Here, we present single-crystal X-ray structures of CheY from Pyrococcus horikoshii (PhCheY) in two different crystal forms, and the protein purification, crystallization and X-ray data collection of CheF (PhCheF). CheA autophosphorylates and subsequently donates the phosphate to CheY, yielding phosphorylated CheY (CheY-P; Garrity & Ordal, 1997; Bischoff et al., 1993; Rudolph & Oesterhelt, 1995; Rudolph et al., 1995). The concentration of CheY-P determines the switching frequency of the flagellum or archaellum, respectively. We observe PhCheY to have a domain-swapped, pseudo-dimeric fold, which may reflect inherent properties of the protein fold but is not likely to be of physiological relevance.

In striking contrast to all of the known CheY structures, PhCheY adopts an open conformation in both crystal forms, with the two subdomains of a given subunit directed away from one another. In both of the two PhCheY structures solved in this study, two polypeptide chains assemble by pairing the N-terminal subdomain of a chain with the C-terminal subdomain of the other chain; i.e. the α3/β4/α4/β5/α5 part of the fold of each subunit packs with the β1/α1/β2/α2 part of the other subunit [Fig. 1(a)]. In the case of the C2 crystal form, there are six molecules in the asymmetric unit. Four of the subunits (A, B, D and F) interact with one another in a dimeric-type domain-swapped assembly. The other two subunits, C and E, interact with their own crystallographic symmetric molecules for the dimeric assembly with swapped domains. Superposition of the N-terminal subdomain among the different subunits A, B, C, D, E and F reveals that the C-terminal domain of subunits B, C, D, E and F undergoes a relative movement of up to 57° with respect to the N-terminal domain. In all cases, the rotational movement of the C-terminal domain was calculated after the initial superposition of the N-terminal domain. The connecting region between the β3–α3 loop is partially disordered for the two subunits C and E. For both crystal forms an unambiguous trace of the electron density in the β3–α3 loop was verified by a feature-enhanced map (FEM; Afonine et al., 2015; shown in Supplementary Fig. S2 for the P2 crystal form). While CheY has been broadly characterized in structure and function, a subdomain swap, as observed in PhCheY, has not been reported before. Therefore, a physiological role for a domain-swapped dimeric PhCheY has to be ruled out.

>[6x]MARVLVVDDAAFMRMLLKKILTQAGHEVVGEASNGKEAVEKYKQLKPDLVTMDIVMPEMDGITAVKEIMKIDPNAKIIMITAVGQEAKVMEALKSGAKGYIVKPFQAQKVIEEVNRVLSS>MGSLAWWKRELFGGWTHFEAVWLLMFLGIQAVVFVFNPDSWLASVAAVTGILCVVFVGKGKISNYLFGLISVSLYAYVSYTFKLYGEMMLNLLVYVPVQFVGFAMWRKHMALGETAETEEVKAKALTVRQWLLVVAASVVGTSVYIEWLHHLGSALPTLDGVTVVVSIVAQVLMILRYREQWALWIVVNILTIS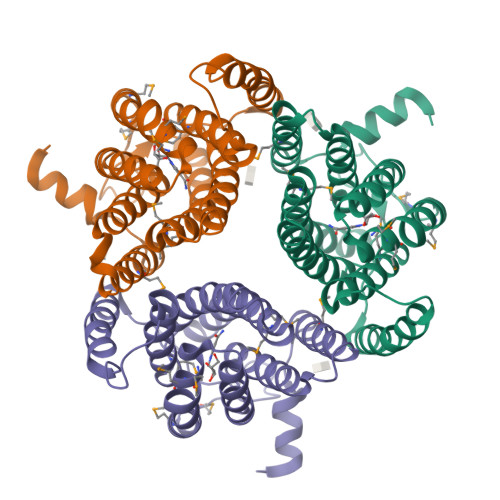LWAVAWFKNGETSLPLLLMYVMYLCNSVYGYINWTKLVKRHSGQHHHHHH[3x]> MESPSSEEEKPLAKMAFTLADRVTEEMLADKAALVVEVVEENYHDAPIVGIAVVNEHGRFFLRPETALADPQFVAWLGDETKKKSMFDSKRAAVALKWKGIELCGVSFDLLLAAYLLDPAQGVDDVAAAAKMKQYEAVRPDEAVYGKGAKRAVPDEPVLAEHLVRKAAAIWELERPFLDELRRNEQDRLLVELEQPLSSILAEMEFAGVKVDTKRLEQMGKELAEQLGTVEQRIYELAGQEFNINSPKQLGVILFEKLQLPVLKKTKTGYSTSADVLEKLAPYHEIVENILHYRQLGKLQSTYIEGLLKVVRPDTKKVHTIFNQALTQTGRLSSTEPNLQNIPIRLEEGRKIRQAFVPSESDWLIFAADYSQIELRVLAHIAEDDNLMEAFRRDLDIHTKTAMDIFQVSEDEVTPNMRRQAKAVNFGIVYGISDYGLAQNLNISRKEAAEFIERYFESFPGVKRYMENIVQEAKQKGYVTTLLHRRRYLPDITSRNFNVRSFAERMA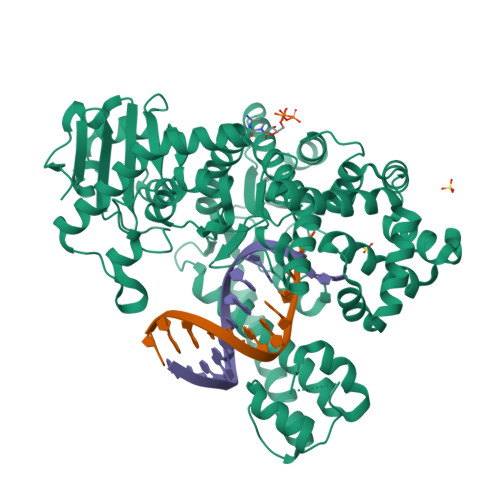MNTPIQGSAADIIKKAMIDLNARLKEERLQAHLLLQVHDELILEAPKEEMERLCRLVPEVMEQAVTLRVPLKVDYHYGSTWYDAK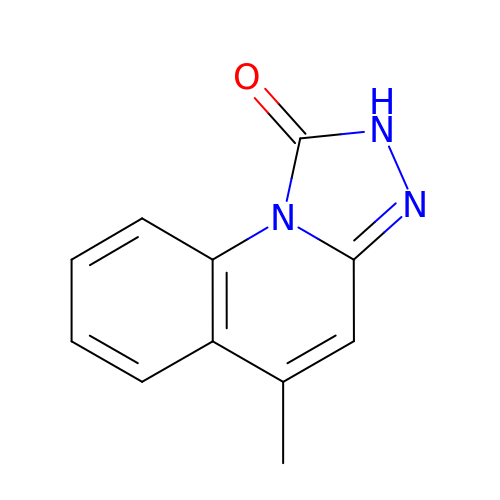5-METHYL[1,2,4]TRIAZOLO[4,3-A]QUINOLIN-1(2H)-ONE | C11 H9 N3 O | VPUMZLVLKCMKFQ-UHFFFAOYSA-N>MFDVIVVGGGPTGLMLAGELRLHGVRVLVLEKETEPTRQSRAQGLHVRSIEVMAQRGLLERFLERGHTVAVGGFFAGLATSWPERLDTAHSYVLAVPQVITEQLLAEHATALGAEIRRGRALVGLRQDEDGVTVDLADGEQLRARYVVGCDGGRSTVRKLLGVAFPGEPSRVETLLGEMEMTASQEELTSVMTEVRKTQQRFGAMPLGDGVFRVVVPAEGVAEDRTASPTLDEFKQQLRAHAGTDFGVHSPRWLSRFGDATRQAERYRVDRVFLAGDAAHIHPPTGGQGLNLGIQDAFNLGWKLAAEVDGWAPEGLLDTYHAERHPVATEVLDNTRAQIQLMSTEPGPQAVRRLMAELVEFENVNRYLIEKITAISVRYDVGEGHELLGRRMRDLALKHGRLYER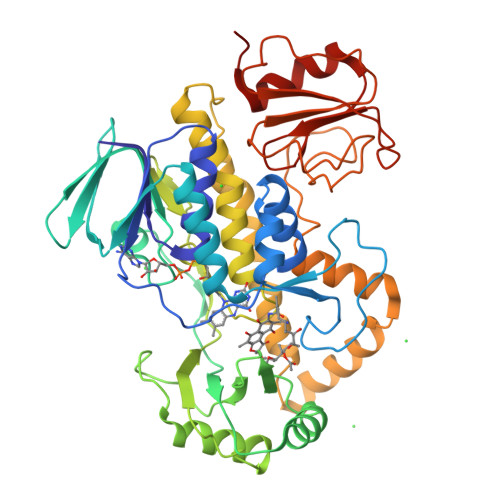MHEGRGLLLDQTGRLSVAGWEDRVDHVVEVSEELDVPAVLLRPDGHVVWAGEDQQELLTRMPAWFGAATAG[3x]> SMAVKSIKVKLRLDDMPEIRAGLWKLHKEVNAGVRYYTEWLSLLRQENLYRRSPNGDGEQECDKTAEECKAELLERLRARQVENGHRGPAGSDDELLQLARQLYELLVPQAIGAKGDAQQIARKFLSPLADKDAVGGLGIAKAGNKPRWVRMREAGEPGWEEEKEKAETRKSADRTADVLRALADFGLKPLMRVYTDSEMSSVEWKPLRKGQAVRTWDRDMFQQAIERMMSWESWNQRVGQEYAKLVEQKNRFEQKNFVGQEHLVHLVNQLQQDMKEASPGLESKEQTAHYVTGRALRGSDKVFEKWGKLAPDAPFDLYDAEIKNVQRRNTRRFGSHDLFAKLAEPEYQALWREDASFLTRYAVYNSILRKLNHAKMFATFTLPDATAHPIWTRFDKLGGNLHQYTFLFNEFGERRHAIRFHKLLKVENGVAREVDDVTVPISMSEQLDNLLPRDPNEPIALYFRDYGAEQHFTGEFGGAKIQCRRDQLAHMHRRRGARDVYLNVSVRVQSQSEARGERRPPYAAVFRLVGDNHRAFVHFDKLSDYLAEHPDDGKLGSEGLLSGLRVMSVALGLRTSASISVFRVARKDELKPNSKGRVPFFFPIKGNDNLVAVHERSQLLKLPGETESKDLRAIREERQRTLRQLRTQLAYLRLLVRCGSEDVGRRERSWAKLIEQPVDAANHMTPDWREAFENELQKLKSLHGICSDKEWMDAVYESVRRVWRHMGKQVRDWRKDVRSGERPKIRGYAKDVVGGNSIEQIEYLERQYKFLKSWSFFGKVSGQVIRAEKGSRFAITLREHIDHAKEDRLKKLADRIIMEALGYVYALDERGKGKWVAKYPPCQLILLAELSEYQFNNDRPPSENNQLMQWSHRGVFQELINQAQVHDLLVGTMYAAFSSRFDARTGAPGIRCRRVPARCTQEHNPEPFPW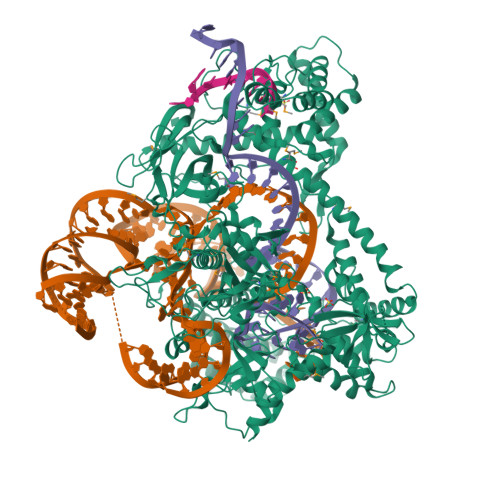WLNKFVVEHTLDACPLRADDLIPTGEGEIFVSPFSAEEGDFHQIHAALNAAQNLQQRLWSDFDISQIRLRCDWGEVDGELVLIPRLTGKRTADSYSNKVFYTNTGVTYYERERGKKRRKVFAQEKLSEEEAELLVEADEAREKSVVLMRDPSGIINRGNWTRQKEFWSMVNQRIEGYLVKQIRSRVPLQDSACENTGDI> MNRFVIADSTLCIGCHTCEAACSETHRQHGLQSMPRLRVMLNEKESAPQLCHHCEDAPCAVVCPVNAITRVDGAVQLNESLCVSCKLCGIACPFGAIEFSGSRPLDIPANANTPKAPPAPPAPARVSTLLDWVPGIRAIAVKCDLCSFDEQGPACVRMCPTKALHLVDNTDIARVSKRKRELTFNTDFGDLTLFQQAQSGEAK;> MSAISLINSGVAWFVAAAVLAFLFSFQKALSGWIAGIGGAVGSLYTAAAGFTVLTGAVGVSGALSLVSYDVQISPLNAIWLITLGLCGLFVSLYNIDWHRHAQVKCNGLQINMLMAAAVCAVIASNLGMFVVMAEIMALCAVFLTSNSKEGKLWFALGRLGTLLLAIACWLLWQRYGTLDLRLLDMRMQQLPLGSDIWLLGVIGFGLLAGIIPLHGWVPQAHANASAPAAALFSTVVMKIGLLGILTLSLLGGNAPLWWGIALLVLGMITAFVGGLYALVEHNIQRLLAYHTLENIGIILLGLGAGVTGIALEQPALIALGLVGGLYHLLNHSLFKSVLFLGAGSVWFRTGHRDIEKLGGIGKKMPVISIAMLVGLMAMAALPPLNGFAGEWVIYQSFFKLSNSGAFVARLLGPLLAVGLAITGALAVMCMAKVYGVTFLGAPRTKEAENATCAPLLMSVSVVALAICCVIGGVAAPWLLPMLSAAVPLPLEPANTTVSQPMITLLLIACPLLPFIIMAICKGDRLPSRSRGAAWVCGYDHEKSMVITAHGFAMPVKQAFAPVLKLRKWLNPVSLVPGWQCEGSALLFRRMALVELAVLVVIIVSRGA;> MSVLYPLIQALVLFAVAPLLSGITRVARARLHNRRGPGVLQEYRDIIKLLGRQSVGPDASGWVFRLTPYVMVGVMLTIATALPVVTVGSPLPQLGDLITLLYLFAIARFFFAISGLDTGSPFTAIGASREAMLGVLVEPMLLLGLWVAAQVAGSTNISNITDTVYHWPLSQSIPLVLALCACAFATFIEMGKLPFDLAEAEQELQEGPLSEYSGSGFGVMKWGISLKQLVVLQMFVGVFIPWGQMETFTAGGLLLALVIAIVKLVVGVLVIALFENSMARLRLDITPRITWAGFGFAFLAFVSLLAA;> MSEEKLGQHYLAALNEAFPGVVLDHAWQTKDQLTVTVKVNYLPEVVEFLYYKQGGWLSVLFGNDERKLNGHYAVYYVLSMEKGHHHHHHHHHHGSTKCWITVRVEVDANKPEYPSVTPRVPAAVWGEREVRDMYGLIPVGLPDERRLVLPDDWPDELYPLRKDSMDYRQRPAPTTDAETYEFINELGDKKNNVVPIGPLHVTSDEPGHFRLFVDGENIIDADYRLFYVHRGMEKLAETRMGYNEVTFLSDRVCGICGFAHSTAYTTSVENAMGIQVPERAQMIRAILLEVERLHSHLLNLGLACHFTGFDSGFMQFFRVRETSMKMAEILTGARKTYGLNLIGGIRRDLLKDDMIQTRQLAQQMRREVQELVDVLLSTPNMEQRTVGIGRLDPEIARDFSNVGPMVRASGHARDTRADHPFVGYGLLPMEVHSEQGCDVISRLKVRINEVYTALNMIDYGLDNLPGGPLMVEGFTYIPHRFALGFAEAPRGDDIHWSMTGDNQKLYRWRCRAATYANWPTLRYMLRGNTVSDAPLIIGSLDPCYSCTDRMTVVDVRKKKSKVVPYKELERYSIERKNSPLK;> MFTFIKKVIKTGTATSSYPLEPIAVDKNFRGKPEQNPQQCIGCAACVNACPSNALTVETDLATGELAWEFNLGHCIFCGRCEEVCPTAAIKLSQEYELAVWKKEDFLQQSRFALCNCRVCNRPFAVQKEIDYAIALLKHNGDSRAENHRESFETCPECKRQKCLVPSDRIELTRHMKEAI;> MSNLLGPRDANGIPVPMTVDESIASMKASLLKKIKRSAYVYRVDCGGCNGCEIEIFATLSPLFDAERFGIKVVPSPRHADILLFTGAVTRAMRSPALRAWQSAPDPKICISYGACGNSGGIFHDLYCVWGGTDKIVPVDVYIPGCPPTPAATLYGFAMALGLLEQKIHARGPGELDEQPAEILHGDMVQPLRVKVDREARRLAGYRYGRQIADDYLTQLGQGEEQVARWLEAENDPRLNEIVSHLNHVVEEARIR

The prototypical hydrogen-producing enzyme, the membrane-bound formate hydrogenlyase (FHL) complex from Escherichia coli, links formate oxidation at a molybdopterin-containing formate dehydrogenase to proton reduction at a [NiFe] hydrogenase. As the pH of the growth medium drops, formate re-enters the cell and synthesis of the formate-hydrogen lyase (FHL) complex is induced. This heptameric membrane-bound complex catalyzes the disproportionation of formate to CO2 and H2 allowing efficient production of hydrogen from biomass, a process that was first described over 100 years ago5. The FHL complex exhibits the characteristic L-shaped structure of the complex I superfamily with membrane-embedded and soluble arms. An electron relay containing eight [4Fe4S] clusters, coordinated by FdhF (A1), HycB (B1-B4), HycF (F1, F2) and HycG (G1), leads from the molybdopterin site to a [NiFe] hydrogenase active site in HycE.

We developed an anaerobic isolation protocol that allowed us to purify a complex exhibiting 20-fold higher hydrogen-uptake activity (6201 ± 1445 s−1) compared to aerobically purified complex from this study (253 ± 164 s−1) and previous studies (2.44 ± 0.62 U mg−1 ≡ 13 s−1). The structure of the anaerobically isolated complex was determined at an average resolution of 2.6 Å. The formate dehydrogenase subunit FdhF, which shows partial occupancy in the aerobically purified complex, was entirely absent in the anaerobically isolated complex in multiple replicates of the purification. In line with its higher hydrogen-uptake activity, the map derived from anaerobically prepared sample had stronger and higher-resolution density for the nickel-iron active site in HycE and the proximal iron-sulfur cluster G1 in HycG. The ND3 loop (HycC TMH15-THM16 loop), β1-β2 loop (HycE β8-β9 loop), NDUFS7 loop (HycG residues 69-80) and the ND1 loop (HycD TMH5-TMH6 loop) are all well-resolved in our anaerobic cryo-EM map and could be modeled with confidence. The structure of anaerobically isolated FHL shows the arginine in a single conformation facing the metal ion. Additional density between the helix HL and TMH7 of HycC could be confidently assigned as cardiolipin (CDL). Arg567, Tyr290, His215, Gln220 and Asn571 of HycC interact with the headgroup of CDL, whereas non-polar residues in the broken helix in TMH7 interact with the alkyl chains. In FHL the Glu193 is too far (4 Å) from Cys531-S to allow direct proton transfer, suggesting that the β1-β2 loop is likely flexible during turnover.> ASPPPGDNGFPAITTASPIESARIGEVKRETKETNVSVKINLDGHGVSDSSTGIPFLDHMLDQLASHGLFDVHVRATGDTHIDDHHTNEDVALAIGTALLKALGERKGINRFGDFTAPLDEALIHVSLDLSGRPYLGYNLEIPTQRVGTYDTQLVEHFFQSLVNTSGMTLHIRQLAGKNSHHIIEATFKAF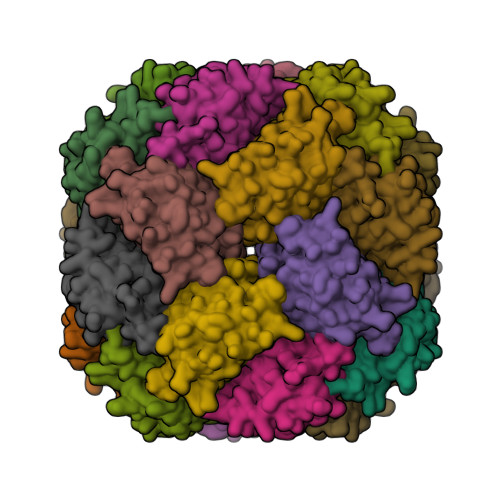ARALRQATESDPRRGGTIPSSKGVLSRS> DVVPHHKLTVNNTKAMKHALERVQLPWKK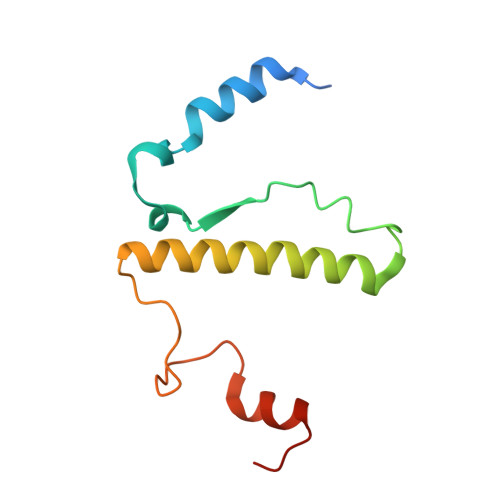HSFQEHQSVTSETNTDEHIKDIYDDTERELAFYKQSLDAVLVARDELKRLKVPFKRPLDYFAEMVKSDEHMDKIKGKLIEE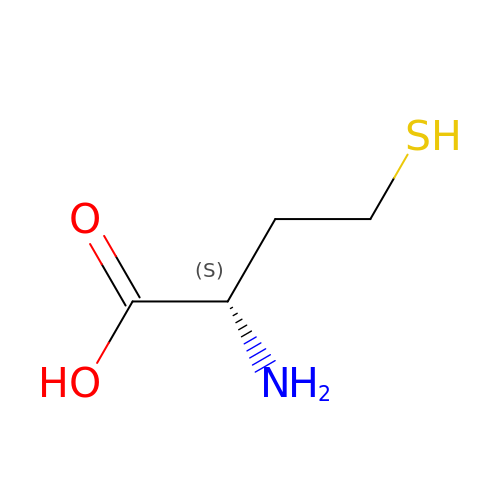2-AMINO-4-MERCAPTO-BUTYRIC ACID | C4 H9 N O2 S | FFFHZYDWPBMWHY-VKHMYHEASA-N To gain further insight into the structural conversions in pore formation, we chose pleurotolysin (Ply), a MACPF protein consisting of two components, PlyA and PlyB, from Pleurotus ostreatus. Previous studies have shown that PlyA binds membranes and is required to recruit the pore-forming MACPF protein PlyB to the membrane surface. PlyA and PlyB together form relatively small and regular pores in liposomes. The membrane attack complex/perforin-like family (MACPF) proteins form the largest superfamily of pore-forming proteins identified to date.

To lock TMH2 to the central core β-sheet of the MACPF domain we identified a second variant PlyBY166C,G266C (TMH2 helix lock) that could be trapped in the prepore state. As with TMH1 lock, addition of reducing agent allows it to continue its trajectory to the pore form. The cryo-EM structure of the TMH2 helix lock prepore revealed a very different picture from the TMH1 lock. The core sheet opening is only 37° ± 11° with some density remaining for TMH1, suggesting that this region remains partly ordered. These data show that the MACPF fold oligomerises without substantial relief of the twist in the core sheet or TMH1 release. As in the TMH1 lock prepore, no density can be seen extending to the membrane surface, consistent with the absence of lytic function. Remarkably, the results reveal that restricting the movement of the top of the TMH2 α-helix prevents unbending of the MACPF core β-sheet. This finding is opposite to expectation, since TMH1 forms an extensive buried interface, whereas TMH2 makes fewer contacts with the domain core sheet. Our findings highlight a critical role of the interface between the top of TMH2 and the surrounding region in controlling sheet opening.

>[2x]AYAQWVIIIIHNVGSKDVKIKNLKPSWGKLHADGDKDTEVSASKYEGTVIKPDEKLQINACGRSDAAEGTTGTFDLVDPADGDKQVRHFYWDCPWGSKTNTWTVSGSNTKWMIEYSGQNLDSGALGTITVDTLKK;> MEAVLSRQAATAEAIGRFQDSSTSVGLVAGSPSTRIRRQADNVVLKSTSQAGDTLNDVIQDPTRRNKLINDNNLLKGIIMGRDGPVPSSRELIVRPDTLRAIINNRATIETTTMEAEFTETLMESNYNSASVKVSAPFITANSEYSESSSFKNTETEKSMYTSSRYLFPQGRIDFTTPDSGFDDVIKLSPQFTSGVQAALAKATGTEKREALQNLFQEYGHVFRTKVHIGGVLSAHTMETFSRSENETEVKQDVKAGLEGAVKGWGGGATAGHGNTQGTITTSQNRKLNVKYIVNGGDYTKIQNTEEWVASTNQSEHWRVIEVTEVTAVADLLPQPIRGQVKDLLKPLLGKWVDVEKVPGLESLPVSVYRPKGAIPAGWFWLGDTADASKALLVKPTLPARSGRNPALTSLHQGSGMTEQPFVDLPQYQYLSTYFGSFAHDTPPGSTLRGLRPDHVLPGRYEMHGDTISTAVYVTRPVDVPFPEDECFDLKSLVRVKLPGSGNPPKPRSALKKSMVLFDSGEK> MGWSCIILFLVATATGVHSGGWSHPQFEKAEAAAKEAAAKEAAAKAAVAEMNPNVNVFVPPRDGFSGPAPRKSKLICEATNFTPKPITVSWLKDGKLVESGFTTDPVTIENKGSTPQTYKVISTLTISEIDWLNLNVYTCRVDHRGLTFLKNVSSTCAASPSTDILTFTIPPSFADIFLSKSANLTCLVSNLATYETLNISWASQSGE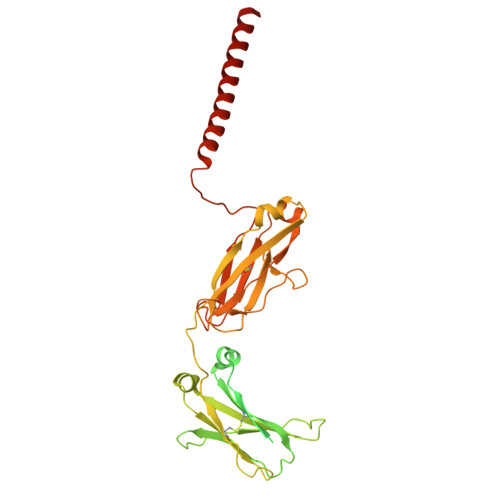PLETKIKIMESHPNGTFSAKGVASVCVEDWNNRKEFVCTVTHRDLPSPQKKFISKPNEVHKHPPAVYLLPPAREQLNLRESATVTCLVKGFSPADISVQWLQRGQLLPQEKYVTSAPMPEPGAPGFYFTHSILTVTEEEWNSGETYTCVVGHEALPHLVTERTVDKSTEGEVNAEEEGFENLWTTASTFIVLFLLSLFYSTTVTLFKVK> MEAAHSKTTEECLAYFGVSETTGLTPDQVKRHLEKYGHNELPAEEGKSLWELVLEQFEDLLVRILLLAACISFVLAWFEEGEETVTAFVEPFVILLILIANAIVGVWQERNAENAIEALKEYEPEMGKVYRADRKSVQRIKARDIVPG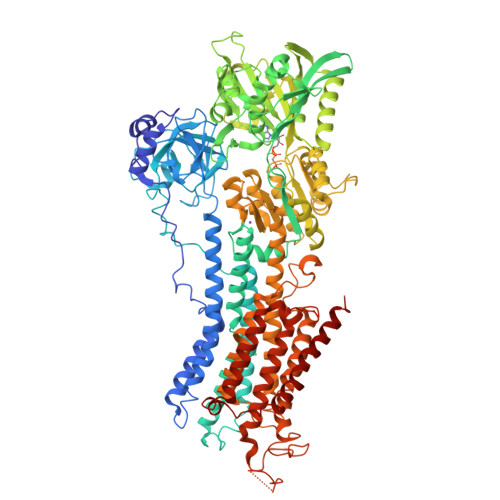DIVEVAVGDKVPADIRILTIKSTTLRVDQSILTGESVSVIKHTEPVPDPRAVNQDKKNMLFSGTNIAAGKAIGIVATTGVGTEIGKIRDQMAATEQDKTPLQQKLDEFGEQLSKVISLICVAVWLINIGHFNDPVHGGSWIRGAIYYFKIAVALAVAAIPEGLPAVITTCLALGTRRMAKKNAIVRSLPSVETLGCTSVICSDKTGTLTTNQMSVCKMFIIDRIDGDLCLLNEFSVTGSTYAPEGEVLKNDKPVRSGQYDGLVELATICALCNDSSLDFNETKGIYEKVGEATETALTTLVEKMNVFNTEVRNLSKVERANACNSVIRQLMKKEFTLEFSRDRKSMSVYCSPAKSRAAVGNKMFVKGAPEGVIDRCNYVRVGTTRVPMTGPVKEKILSVIKEWGTGRDTLRCLALATRDTPPKREEMVLDDSTKFMEYETDLTFVGVVGMLDPPRKEVMGSIQLCRDAGIRVIMITGDNKGTAIAICRRIGIFGENEDVADRAYTGREFDDLPLAEQREACRRACCFARVEPTHKSKIVEYLQSFDEITAMTGDGVNDAPALKKAEIGIAMGSGTAVAKTASEMVLADDNFSTIVAAVEEGRAIYNNMKQFIRYLISSNVGEVVCIFLTAALGLPEALIPVQLLWVNLVTDGLPATALGFNPPDLDIMDRPPRTPKEPLISGWLFFRYMAIGGYVGAATVGAAAWWFLYAEDGPHVTYSQLTHFMKCSEHSPDFEGVDCEVFEAPQPMTMALSVLVTIEMCNALNSLSENQSLVRMPPWVNIWLVGSIGLSMSLHFLILYVDPLPMIFKLQALDLYHWLMVLKISLPVIGLDEILKFVARNYLE>MNPAAEAEFNILLATDSYKVTHYKQYPPNTSKVYSYFECREKKTENSKLRKVKYEETVFYGLQYILNKYLKGKVVTKEKIQEAKDVYKEHFQDDVFNEKGWNYILEKYDGHLPIEIKAVPEGFVIPRGNVLFTVENTDPECYWLTNWIETILVQSWYPITVATNFREQKKILAKYLLETSGNLDGLEYKLHDFGYRGVSSQETAGIGASAHLVNFKGTDTVAGLALIKKYYGTKDPVPGYSVPAAEHSTITAWGKDHEKDAFEHIVTQFSSVPVSVVSDSYDIYNACEKIWGEDLRHLIVSRSTQAPLIIRPDSGNPLDTVLKVLEILGKKFPVTENSKGYKLLPPYLRVIQGDGVDINTLQEIVEGMKQKMWSIENIAFGSGGGLLQKLTRDLLNCSFKCSYVVTNGLGINVFKDPVADPNKRSKKGRLSLHRTPAGNFVTLEEGKGDLEEYGQDLLHTVFKNGKVTKSYSFDEIRKNAQLN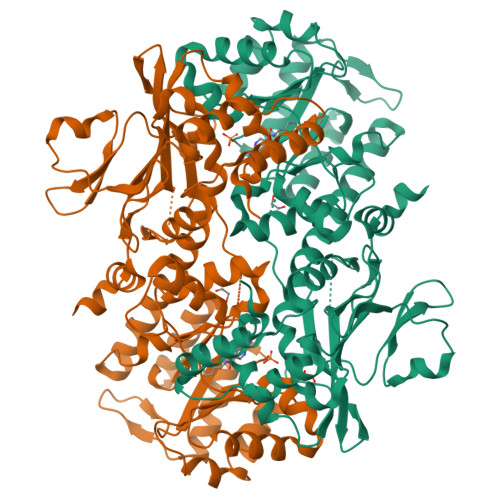IELEAAHHLEHHHHHHHH[2x]The exo-β-1,3-galactanase is a glycoside hydrolase from the basidiomycete Phanerochaete chrysosporium (Pc1,3Gal43A), which specifically cleaves AGPs. In this context, exo-β-1,3-galactanase (EC 3.2.1.145) specifically cleaves the nonreducing end β-1,3–linked galactosyl linkage of β-1,3-galactans to release d-galactose (Gal). In this study, we solved the apo and liganded structures of Pc1,3Gal43A, which reveal a glycoside hydrolase family 43 subfamily 24 (GH43_sub24) catalytic domain together with a carbohydrate-binding module family 35 (CBM35) binding domain. The N-terminal catalytic domain consists of a five-bladed β-propeller (Gln21–Gly325), as in other GH clan-F enzymes, and the C-terminal domain (PcCBM35) takes a β-jellyroll fold (Thr326–Tyr448) structure, as in previously reported CBM35s.

The Gal3 molecule co-crystallized with the E208Q mutant occupies subsites −1, +1, and +2 of the catalytic site, from the nonreducing end to the reducing end. Gal−1 is located at the bottom of the catalytic cavity, and Gal+1 and Gal+2 extend linearly outwards. Gal−1 adopts a 1S3 skew boat conformation and interacts with many residues via hydrogen bonds and hydrophobic interactions. As shown in Fig. 2 (B and C), the C-2 hydroxyl group of Gal−1 forms hydrogen bonds with NH2 of Arg103 and with OE1 of Gln263 via water. Notably, Trp229 supports the flat C3-C4-C5-C6 structure of Gal−1, and Tyr126 recognizes the C-6 methylol and C-4 hydroxyl groups, whereas Glu102 recognizes the C-3 hydroxyl and C-4 hydroxyl groups. In Gal+1, the C-2 hydroxyl group forms a hydrogen bond with NE2 of Gln208 and N of Gly228, whereas O5 forms a hydrogen bond with ND2 of Asn180, and C-6 hydroxyl group forms a hydrogen bond with OD1 of Asn179 via water. In Gal+2, the C-2 and C-4 hydroxyl groups form hydrogen bonds with OG1 of Thr226 and ND2 of Asn180, respectively. The C-6 methylol group of Gal−1 is exposed to the solvent, so that the side chain can be accommodated externally. E208Q_Gal3 showed small movements of Trp229, but other structures showed much larger fluctuations. At the catalytic site, Gal−1 is anchored in the appropriate position, and Gal+2 appears to fluctuate in a planar fashion as it interacts with the surrounding residues.

> QNQIVSGAAWTDTAGNTIQAHGAGILQVGSTFYWFGEDKSHNSALFKAVSCYTSSDLVNWSRQNDALSPIAGTMISTSNVVERPKVIFNQKNSEYVMWFHSDSSNYGAAMVGVATAKTPCGPYTYKGSFKPLGADSRDESIFQDDDSAQTAYLLYASDNNQNFKISRLDANYYNVTAQVSVMNGATLQAPGIVKHNGEYFLIASHTSGWAPNPNKWFSASSLAGPWSAQQDIAPSATRTWYSQNAFDLPLGSNAIYMGDRWRPSLLGSSRYIWYPLDFSSGAPQIVHADVWSVNVQAGTYSVASGTSYEAENGQRGGSSTILSGSGFSGGKAVGYLGHGGTVTINNVQSNGGSHWVALYFANGDSTYRNVTVSVNGGPSVLVDQPDSGGGNVVISVPVKLNLNSGENSITFGSGQSNYAADLDKIIVY> ATYSTVPKIAFYAGLKRQHEGYEVLKFDDVVTNLGNHYDPTTGKFTCSIPGIYFFTYHVLMRGGDGTSMWADLCKNNQVRASAIAQAADQNYDYASNSVVLHLEPGDEVYIKL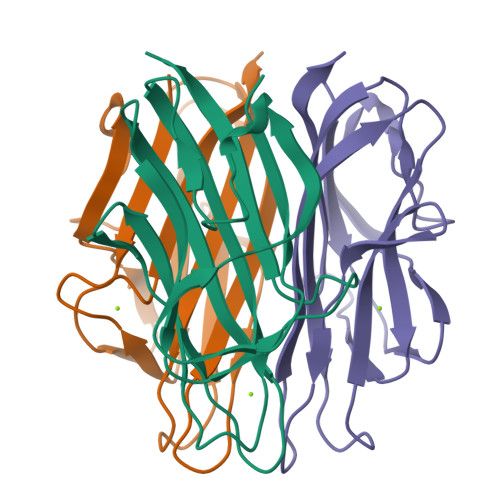DGGKAHGGNNNKYSTFSGFIIYAD>[8x]GSLAPMFERLSTESVQEQLPYSVTLISMPATTEGRRGFSVSVESASSNYATTVQVKEVNRMHISPNNRNAIHPGDRILEINGTPVRTLRVEEVEDAISQTS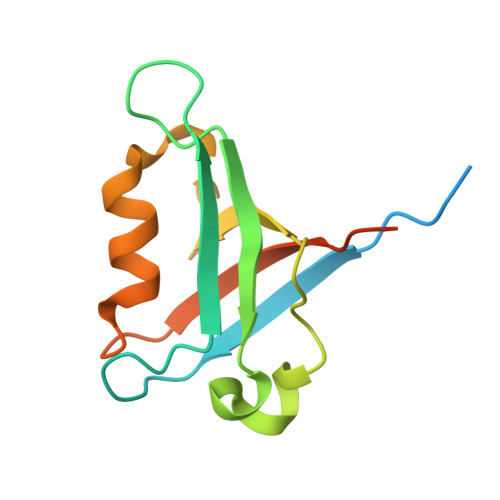QTLQLLIEHDPVSQRLDQLRLE> GPGLKQKIVIKVAMEGNNCRSKAMALVASTGGVDS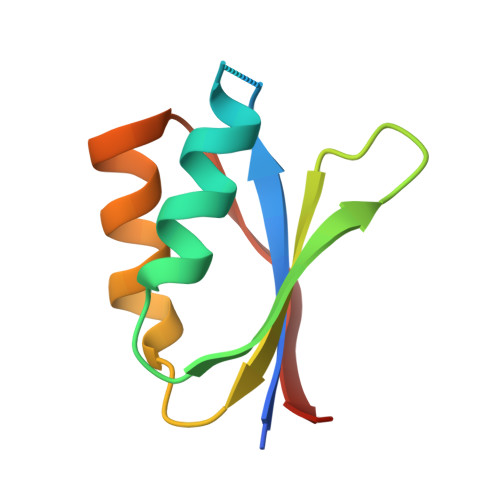VALVGDLRDKIEVVGYGIDPIKLISALRKKVGDAELLQVSQANKD>[2x]MEKILIFGHQNPDTDTICSAIAYADLKNKLGFNAEPVRLGQVNGETQYALDYFKQESPR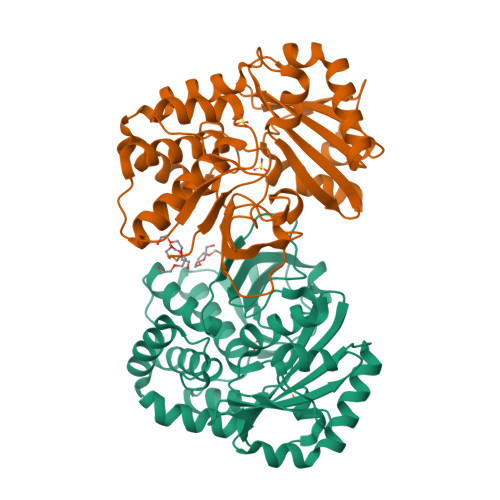LVETAANEVNGVILVDHNERQQSIKDIEEVQVLEVIDHHRIANFETAEPLYYRAEPVGCTATILNKMYKENNVKIEKEIAGLMLSAIISDSLLFKSPTCTDQDVAAAKELAEIAGVDAEEYGLNMLKAGADLSKKTVEELISLDAKEFTLGSKKVEIAQVNTVDIEDVKKRQAELEAVISKVVAEKNLDLFLLVITDILENDSLALAIGNEAAKVEKAFNVTLENNTALLKGVVSRKKQVVPVLTDAMAE>[2x]MGSSHHHHHHSSGENLYFQGSQIHVDTMKVINDPIHGHIELHPLLVRIIDTPQFQRLRYIKQLGGGYYVFPGASHNRFEHSLGVGYLAGCLVHALGEKQPELQISERDVLCVQIAGLCHDLGHGPFSHMFDGRFIPLARPEVKWTHEQGSVMMFEHLINSNGIKPVMEQYGLIPEEDIYFIKEQIVGPLESPVEDSLWPYKGRPENKSFLYEIVSNKRNGIDVDKWDYFARDCHHLGIQNNFDYKRFIKFARVCEVDNELRICARDKEVGNLYDMFHTRNSLHRRAYQHKVGNIIDTMITDAFLKADDYIEITGAGGKKYRISTAIDDMEAYTKLTDNIFLEILYSTDP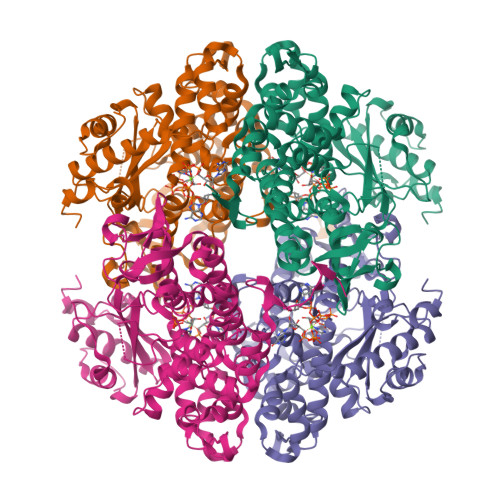KLKDAREILKQIEYRNLFKYVGETQPTGQIKIKREDYESLPKEVASAKPKVLLDVKLKAEDFIVDVINMDYGMQEKNPIDHVSFYCKTAPNRAIRITKNQVSQLLPEKFAEQLIRVYCKKVDRKSLYAARQYFVQWCADRNFTKPQDGDVIAPLITPQKKEWNDSTSVQNPTRLREASKSRVQLFKDDPM>[4x]MAYAQWVIIIIHNVGSKDVKIKNLKPSWGKLHADGDKDTEVSASKYEGTVIKPD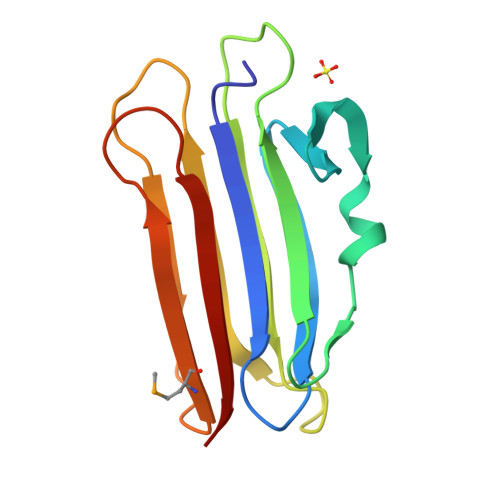EKLQINACGRSDAAEGTTGTFDLVDPADGDKQVRHFYWDCPWGSKTNTWTVSGSNTKWMIEYSGQNLDSGALGTITVDTLKKGN>[6x]MAKKTSSKGKLPPGPRPLPLLGNLLQMDRRGLLKSFLRFREKYGDVFTVHLGPRPVVMLCGVEAIREALVDKAEAFSGRGKIAMVDPFFRGYGVIFANGNRWKVLRRFSVTTMRDFGMGKRSVEERIQEEAQCLIEELRKSKGALMDPTFLFQSITANIICSIVFGKRFHYQDQEFLKMLNLFYQTFSLISSVFGQLFELFSGFLKHFPGAHRQVYKNLQEINAYIGHSVEKHRETLDPSAPRDLIDTYLLHMEKEKSNAHSEFSHQNLNLNTLSLFFAGTETTSTTLRYGFLLMLKYPHVAERVYREIEQVIGPHRPPELHDRAKMPYTEAVIYEIQRFSDLLPMGVPHIVTQHTSFRGYIIPKDTEVFLILSTALHDPHYFEKPDAFNPDHFLDANGALKKTEAFIPFSLGKRICLGEGIARAELFLFFTTILQNFSMASPVAPEDIDLTPQECGVGKIPPTYQIRFLPRHHHH

The cytochrome P450 (CYP) enzymes found on the membrane of the endoplasmic reticulum are a superfamily of heme-containing monooxygenases involved in the biotransformation of drugs and other xenobiotics. CYP2B6 shares at least 75% amino acid sequence identity with other members of the subfamily, constitutes up to 10% of the functional CYP enzymes in human liver, and is responsible for the metabolism of 10–12% of all drugs currently available on the market. CYP2B6 is the major catalyst of efavirenz oxidation and conversion to the most abundant metabolite 8-hydroxyefavirenz, which is then glucuronidated. CYP2B6 also plays an important role in the bioactivation of many procarcinogens and environmental toxicants such as polychlorinated biphenyls, chlorpyrifos, and polybrominated diphenyl ethers.

The CYP2B6 used for expression, purification, structure determination and any other work in this study includes engineered mutations Y226H and K262R in the N-terminally truncated and modified construct with a His-tag at the C-terminus. Because of the relatively low-affinity binding of efavirenz itself, the 2-desoxo-2-methyl analog that demonstrated high-affinity binding (KS = 0.21 ± 0.06 μM) was used for the structural studies reported here. The 2-desoxo-2-methyl analog contains a methyl group in place of the carbonyl oxygen in efavirenz. Interestingly, the chlorine of the efavirenz analog 2-desoxo-2-methyl (abbreviated as I for convenience) forms a π bond with F108 in a similar fashion to that illustrated in our recent study using monoterpenes. The orientation of the methyl group towards the heme-iron corroborates the putative metabolic transformation at the oxazinone ring shown more recently by Cox and Bumpus. The trifluoro group was located near the I101 and F115 side chains, whereas the cyclopropyl group was placed between the side chains of F206 and T302. The CYP2B6-I structure adopted a closed conformation that is similar to the α-pinene complex. The phenyl ring of F297 rotates ~90° to make room for the chloro group of the analog. The F297 side chain is pushed away by more than 2 Å, in contrast to the amlodipine complex, and is likely to accommodate the chlorine group of I that is involved in the π-interactions with the F108 aromatic ring. And observed in the current structure, the R262 side chain may play a crucial role in hydrogen bonding with neighboring helices, which could impact the enzyme structure and function.5-[(3aS,4R,6aR)-2-oxohexahydro-1H-thieno[3,4-d]imidazol-4-yl]-N-(2-oxopropyl)pentanamide 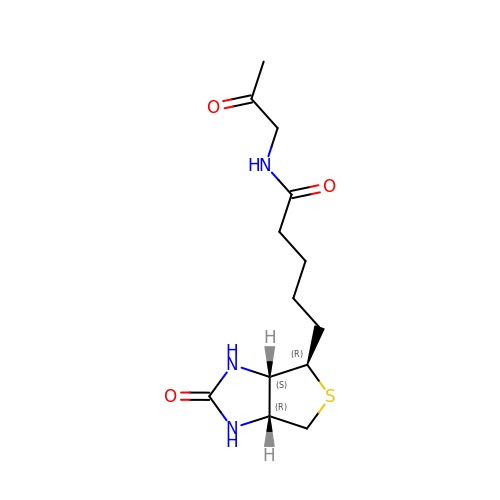| C13 H21 N3 O3 S | NVGARBFYWDPYAF-UMNHJUIQSA-N> METKPRTPVLWLHGLECTCCSESFIRSAHPLAKDVVLSMISLDYDDTLMAAAGHQAEAILEEIMTKYKGNYILAVEGNPPLNQDGMSCIIGGRPFIEQLKYVAKDAKAIISWGSCASWGCVQAAKPNPTQA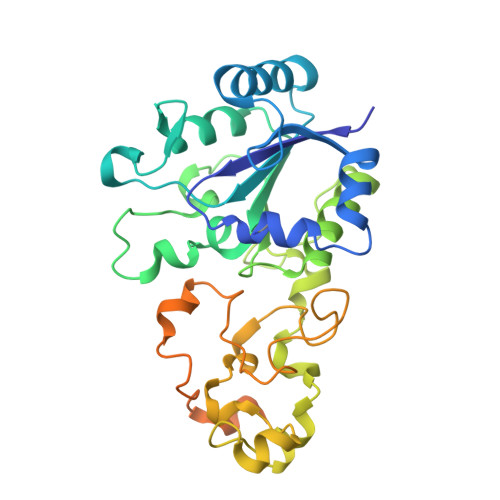TPVHKVITDKPIIKVPGCPPIAEVMTGVITYMLTFDRIPELDRQGRPKMFYSQRIHDKCYRRPHFDAGQFVEEWDDESARKGFCLYKMGCKGPTTYNACSTTRWNEGTSFCIQSGHGCIGCSEDGFWDKGSFYDRLTGISQFGVEANADKIGGTASVVVGAAVTAHAAASAIKRASKKNETSGSEHRSAWSHPQFEK> GPHMASMVKKVNNPLKIDYQNGIIENRLLQIRNFKDVNTPKLINVWSIRIDPRDSKKVIELIRNDFQKNDPVSLRHLKRIRKDIETSTLEVVLCSKEYICDEGEINNKLKSIWVGTKKYELSDDIEVPEFAPSTKELNNAWSVKYWPLIWNGNPNDQILNDYKIDMQEVRNELSRASTLSVKMATAGKQFP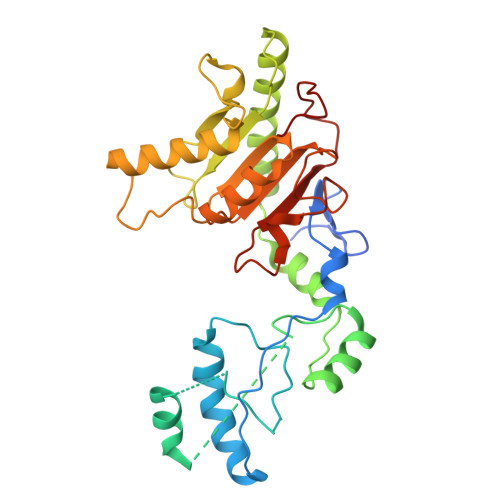MVSVFVDPSRKKDKVVAEDGRNCENSLPIDHSVMVGIRAVGERLREGVDEDANSYLCLDYDVYLTHEPCSMCSMALIHSRVRRVVFLTEMQRTGSLKLTSGDGYCMNDNKQLNSTYEAFQWIGEEYPVGQVDRDVCC>MTDFTPETPVLTPIRDHAAELAKAEAGVAEMAAKRNNRWYPKYHIASNGGWINDPNGLCFYKGRWHVFYQLHPYGTQWGPMHWGHVSSTDMLNWKREPIMFAPSLEQEKDGVFSGSAVIDDNGDLRFYYTGHRWANGHDNTGGDWQVQMTALPDNDELTSATKQGMIIDCPTDKVDHHYRDPKVWKTGDTWYMTFGVSSADKRGQMWLFSSKDMVRWEYERVLFQHPDPDVFMLECPDFSPIKDKDGNEKWVIGFSAMGSKPSGFMNRNVSNAGYMIGTWEPGGEFKPETEFRLWDCGHNYYAPQSFNVDGRQIVYGWMSPFVQPIPMEDDGWCGQ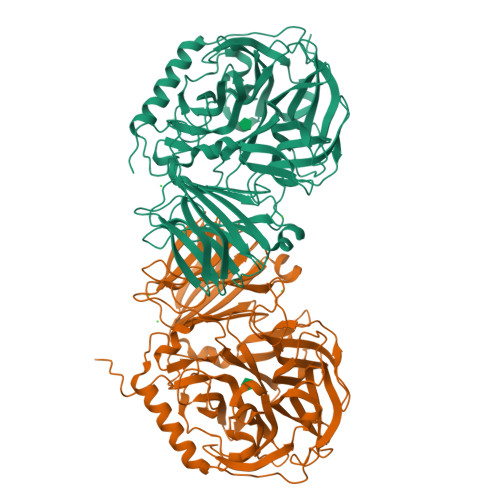LTLPREITLGDDGDVVTAPVAEMEGLREDTLDHGSVTLDMDGEQIIADDAEAVEIEMTIDLAASTAERAGLKIHATEDGAYTYVAYDGQIGRVVVDRQAMANGDRGYRAAPLTDAELASGKLDLRVFVDRGSVEVYVNGGHQVLSSYSYASEGPRAIKLVAESGSLKVDSLKLHHMKSIGLELEHHHHHH[2x]> SAEACGYSDRVAQLTLGNSTITTQEAANIVVAYGRWPSGLRDTDATAVDKPTQPGVSAERFYTLPSVQWTTSF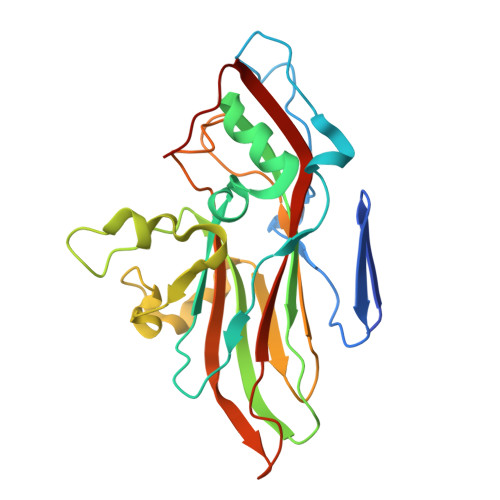TGHYWKLPDALSDLGLFGQNLQFHYLYRGGWAIHVQCNATKFHQGTLLVVAVPEHKIQAQSNPSFGRTNPGEAGAACQFPFTFEDGTALGNALIYPHQWINLRTNNSATLVLPYVNAIPMDSGIKHNNWTLLVIPIVPLEYAVGATTFVPITVTIAPMCTEYNGLRAAVTQ>GDIAIYWGQNGGEGTLASTCDTGRYAYVIVSFVTTFGN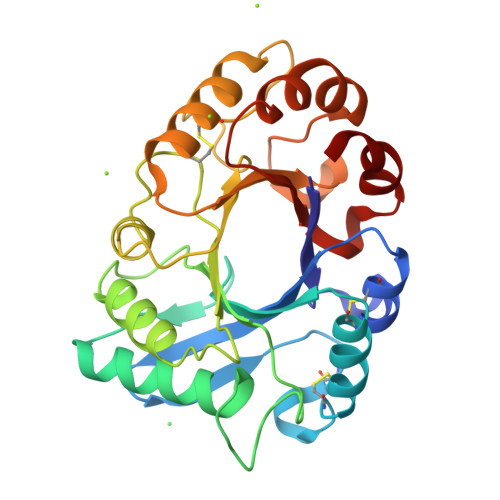FRAPVVNLAGHCDPAAGTCTGLSDEIRSCQGKDIKVLMSIGGGAGDYSLVSEADADNFADYLWNNFLGGQSSSRPLGDAVLDGIDFDIELGTTTFYDTLARALSSRSTQAAKVYLTAAPQCPHPDSHLDAALNTGLFDNVWIQFYNNPLAQCQYSSGNTNDILSSWNTWTSSTTAGKIFLGLPAAPEAAGSGYIPPDVLTGQILPQIKTSAKYGGVMLYSKFYDTTYSTTIKDQV[4x]>GHMSTQAAMTTTERWQKIQGRAPDPIFELAKRAAAAKGPKANLVIGAYRDEQGLPYPLRVVRKAEQLLLDMNLNYEYL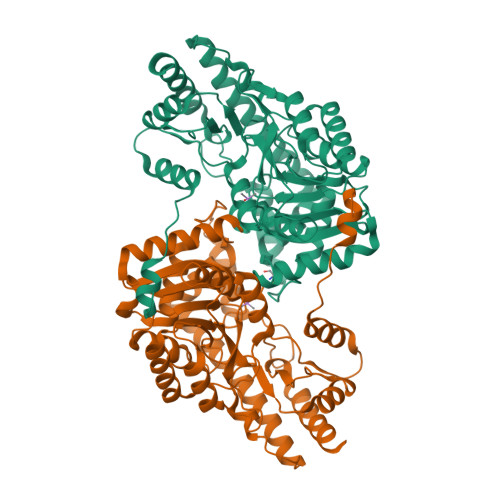PISGYQPFIDEAVKMTYGDTVELENLVAVQTLSGTGALSLGAKLLTHVFDAEKTPIYLADPTWPNHYSIVKAAGWKDIRTYAYYDHKTLGLDFEGMKKDILAAPDGSVFLLHQCAHNPTGVDPSQEQWNEIASLMLAKHHQVFFDSAYQGYASGSLDTDAYAARLFARRGIEVLLAQSFSKNMGLYSERAGTLSLLLKDKTKRADVKSVMDSLIRAEYTCPPAHGARLAHLILSNNELRKEWEAELSAMAERIRTMRRTVYDELLRLQTPGRWEHVINQIGMFSFLGLSKEQCEYCQNHNIFITLSGRANIAGLTHETALMLAQTINDAVRNVNRE[2x]> MGRFIFVSFGL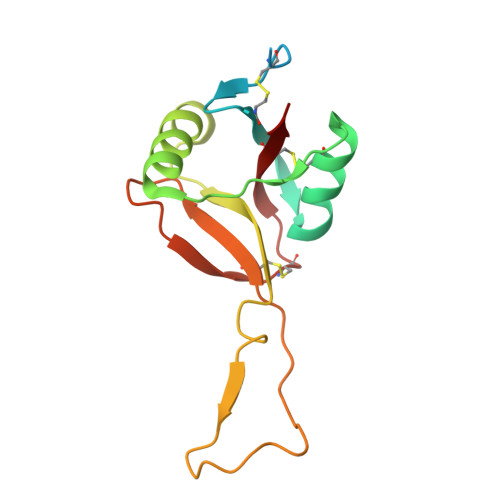LVVFLSLRGTGAGFCCPLRWSSYEGHCYLVVKEKKTWDDAEKFCTEQRKGGHLVSVHSREEADFLVHLAYPILDLSLIWMGLSNMWNDCKREWSDGTKLDFKAWAKTSDCLIGKTDGDNQWLNMDCSKKHYFVCKFKL> IVGGQECKDGECPWQALLINEENEGFCGGTILSEFYILTAAHCLYQAKRFKVRVGDRNTEQEEGGEAVHEVEVVIKHNRFTKETYDFDIAVLRLKTPITFRMNVAPACLPERDWAESTLMTQKTGIVSGFGRTHEKGRQSTRLKMLEVPYVDRNSCKL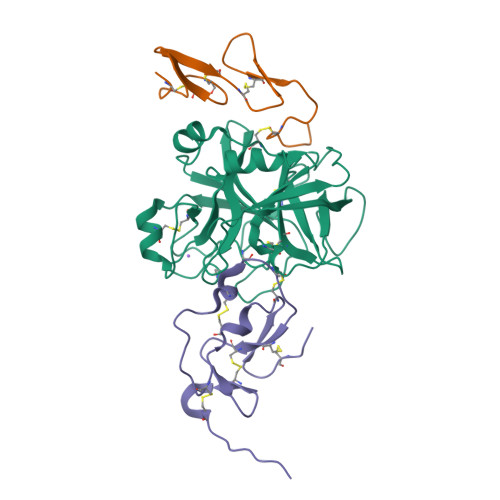SSSFIITQNMFCAGYDTKQEDACQGDSGGPHVTRFKDTYFVTGIVSWGEGCARKGKYGIYTKVTAFLKWIDRSMKTR;> TRKLCSLDNGDCDQFCHEEQNSVVCSCARGYTLADNGKACIPTGPYPCGKQTLE;> RKAYPECGENEWLDDCGTQKPCEAKCNEEPPEEEDPICRSRGCLLPPACVCKDGFYRDTVIGDCVREEECDQHEIIHV Curli are functional amyloids that play critical roles in biofilm formation and adhesion in many Enterobacteriaceae. Two outer membrane proteins, CsgG and CsgF, form the core apparatus for secretion and assembly of the curli structural subunits. In this work, we show that CsgF forms a stable complex with CsgG via a 1:1 stoichiometry by lining the extracellularly faced lumen of the nonameric CsgG channel via its N-terminal 27 residues, creating a secretion channel with 2 constriction regions for curli subunit secretion. The free C-terminal domain of CsgF recruits and binds the secreted nucleator CsgB, creating a growth point for further addition of CsgA subunits.

To obtain the structure of the CsgG-CsgF complex, the full-length E. coli csgG and csgF genes were co-expressed in E. coli strain BL21 (DE3), and the purified CsgG-CsgF complex was applied to the glow-discharged GIG R1/1(Cu) grid for cryo-EM specimen preparation. We collected cryo-EM images for the sample, and cryo-EM structure determination using multiple rounds of three-dimensional (3D) classification and refinement resulted in a density map with an overall resolution of 3.6 Å (S1A, S1B). Overall, the structure of the CsgG-CsgF complex reveals that CsgF forms a 1:1 stable complex with CsgG via its N-terminus (residues 20–53 of the full-length CsgF), yet its C-terminus including residues 54–138 is invisible in the map due to flexibility. The nonameric CsgG structure in the CsgG-CsgF complex is almost identical to the crystal structure of the nonameric CsgG with a root-mean-square deviation (RMSD) of approximately 0.5 Å for all 1,854 aligned Cα atoms. By contrast, the visible CsgG-bound CsgF fragment adopts a loop-helix-loop conformation, distinct from its nuclear magnetic resonance (NMR) structure but consistent with the result of secondary structural prediction. Strikingly, the nonameric CsgG-CsgF complex forms a secretion pore with 2 constriction regions. In addition to the constriction region that is lined with 3 stacked 9-residue rings consisting of either Tyr66, Asn70, or Phe71 of CsgG, the CsgG-bound CsgF adds another constriction region to the CsgG channel. This pore eyelet is formed by 9 Asn36 residues, contributed by each CsgF molecule, with a diameter of approximately 14.8 Å. From the structure of the CsgG-CsgF complex and the isolated CsgF NMR structure, we learned that the orientation between the N-terminus and the C-terminal domain of CsgF is not conformationally fixed, which made the C-terminus of CsgF invisible in the cryo-EM structure.

>MQRLFLLVAVMLLSGCLTAPPKEAARPTLMPRAQSYKDLTHLPAPTGKIFVSVYNIQDETGQFKPYPASNFSTAVPQSATAMLVTALKDSRWFIPLERQGLQNLLNERKIIRAAQENGTVAINNRIPLQSLTAANIMVEGSIIGYESNVKSGGVGARYFGIGADTQYQLDQIAVNLRVVNVSTGEILSSVNTSKTILSYEVQAGVFRFIDYQRLLEGEVGYTSNEPVMLCLMSAIETGVIFLINDGIDRGLWDLQNKAERQNDILVKYRHMSVPPES[9x];>[9x]MRVKHAVVLLMLISPLSWAGTMTFQFRNPNFGGNPNNGAFLLNSAQAQNSYKDPSYNDDFGIETPSALDNFTQAIQSQILGGLLSNINTGKPGRMVTNDYIVDIANRDGQLQLNVTDRKTGQTSTIQVSGLQNNSTDF> SFQKIYSPTQLANAMKLVRQQNGWTQAELAKKIGIKQATISNFENNPDN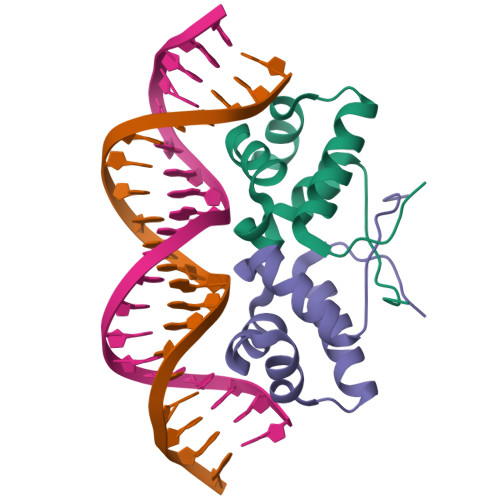TTLTTFFKILQSLELSMTLCDAK>MNKKELIDRVAKKAGAKKKDVKLILDTILETITEALAKGEKVQIVGFGSFEVRKAAARKGVNPQT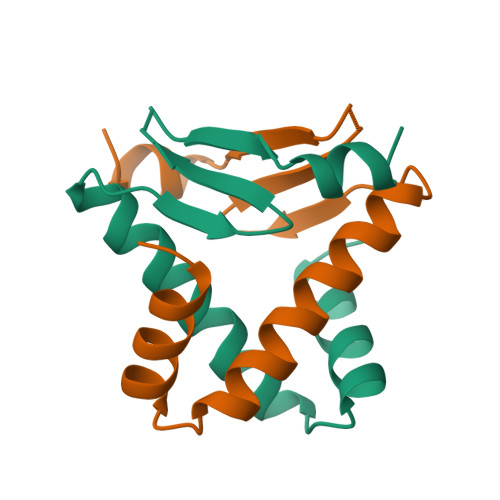RKPITIPERKVPKFKPGKALKEKVK[2x]> IVGGYTCAANSIPYQVSLNSGSHFCGGSLINSQWVVSAAHCYKSRIQVRLGEHNIDVLEGNEQFINAAKIITHPNFNGNTLDNDIMLIKLSSP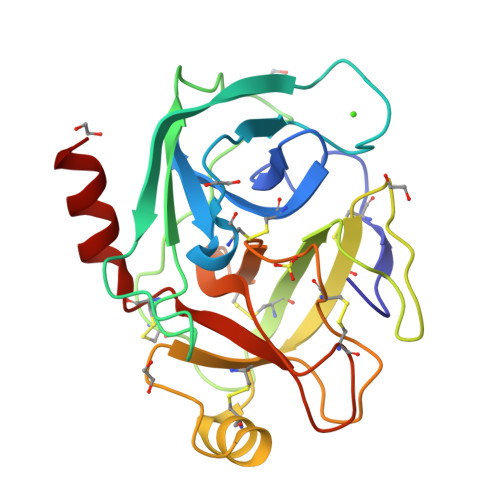ATLNSRVATVSLPRSCAAAGTECLISGWGNTKSSGSSYPSLLQCLKAPVLSNSSCKSSYPGQITGNMICVGFLQGGKDSCQGDSGGPVVCNGQLQGIVSWGYGCAQKNKPGVYTKVCNYVNWIQQTIAAN>[2x]SLRANDAPIVLLHGFTGWGREEMFGFKYWGGVRGDIEQWLNDNGYRTYTLAVGPLSSNWDRACEAYAQLVGGTVDYGAAHAAKHGHARFGRTYPGLLPELKRGGRIHIIAHSQGGQTARMLVSLLENGSQEEREYAKAHNVSLSPLFEGGHHFVLSVTTIATPHDGTTLVNMVDFTDRFFDLQKAVLEAAAVASNVPYTSQVYDFKLDQWGLRRQPGESFDHYFERLKRSPVWTSTDTARYDLSVSGAEKLNQWVQASPNTYYLSFSTERTYRGALTGNHYPELGMNAFSAVVCAPFLGSYRNPTLGIDERWLENDGIVNTVSMNGPKRGSSDRIVPYDGTLKKGVWNDMGTYNVDHLEIIGVDPNPSFDIRAFYLRLAEQLASLQP

Most lipases contain a lid domain controlling access to the active site. The interaction of the enzyme with the lipid aggregates induces the displacement of the lid, which makes the active site accessible to individual substrate molecules and increases the catalytic activity. Here, we report on the effect of an ion pair network on the stability of T1 lipase by introducing an additional ion pair at the inter-loop and the intra-loop. In addition, we elucidated the structure of D311E lipase to identify the additional interactions that govern the stability of this mutant.

The X-ray structure of D311E lipase (2.1 Å) showed a typical α/β hydrolase canonical fold consisting of 11 β-strands and 13 α-helices. The Ser113, Asp317 and His358 were assigned as the catalytic triad. Compared to BTL2 lipase, this crystal lipase was solved in closed conformation at high resolution (2.1 Å) using in-house X-ray diffractometer. In D311E lipase, the ion pair network was composed of five amino acid residues (Arg 274, Thr 278, Gly 279, Arg 303 and Glu 311) connected by seven ion pairs. In D311E lipase, the distances from these ion pairs were between 2.5 Å and 5.2 Å. In contrast, the distances of ion pair involved in T1 lipase were longer than those in D311E lipase. The Glu 311 and Gly 279 were connected by one hydrogen bond and linked to each other at an α-helix and a band region. T1 lipase (circle), K344R lipase (triangle) and D311E lipase (square) showed different Tm, which were 68.52 °C, 68.54 °C and 70.59 °C, respectively. The t1/2 of D311E lipase at 60 °C and 70 °C was 110 min and up to 12 h, respectively. The improved stability of D311E lipase was due to additional inter-loop interactions, which were indicated by the atomic details of D311E lipase with the observed additional ion pair and hydrogen bond interactions.> SANNPWTGFQIFLSPYY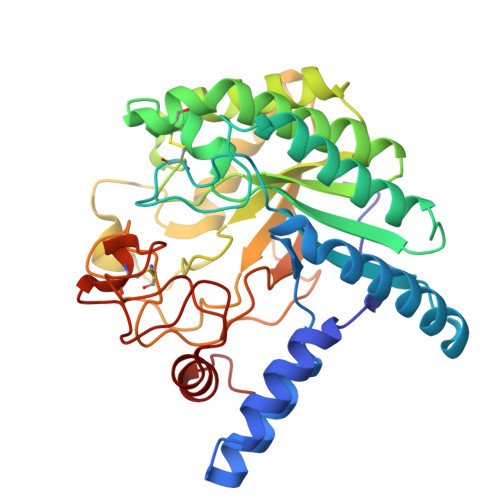ANEVAAAAKQITDPTLSSKAASVANIPTFTWLDSVAKIPDLGTYLASASALGKSTGTKQLVQIVIYDLPDRNCAAKAVNGEFSIANNGQANYENYIDQIVAQIQQFPDVRVVAVIEPDSLANLVTNLNVQKCANAKTTYLASVNYALTNLAKVGVYMYMDAGHAGWLGWPANLSPAAQLFTQVWQNAGKSPFIKGLATNVANYNALQAASPDPITQGNPNYDEIHYINALAPLLQQAGWDATFIVDQGRSGVQNIRQQWGDWCNIKGAGFGTRPTTNTGSQFIDSIVWVKPGGESDGTSNSSSPRYDSTCSLPDAAQPAPEAGTWFQAYFQTLVSAANPPL> GRCYKSRPP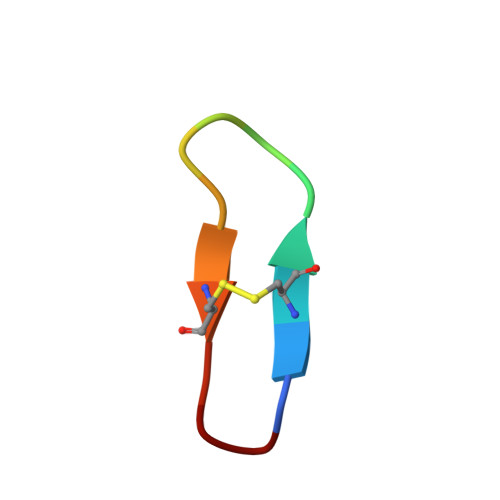ICFPN>[2x]MTIYVVTPTYARLVQKAELVRLSQTLSLVPRLHWLLVEDAEGPTPLVSGLLAASGLLFTHLVVLTPKAQRLREGEPGWVHPRGVEQRNKALDWLRGRGGAVGGEKDPPPPGTQGVVYFADDDNTYSRELFEEMRWTRGVSVWPVGLVGGLRFEGPQVQDGRVVGFHTAWEPSRPFPVDMAGFAVALPLLLDKPNAQFDSTAPRGHLESSLLSHLVDPKDLEPRAANCTRVLVWHTRTE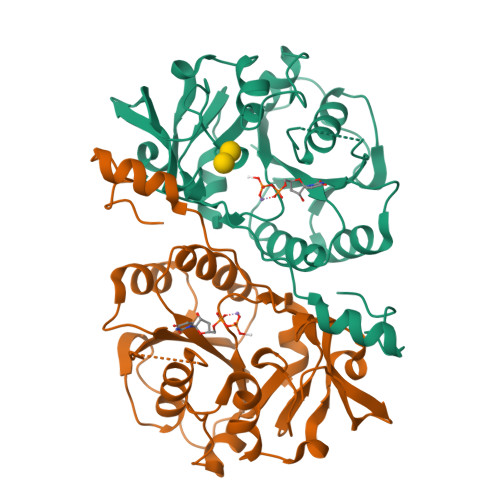KPKMKQEEQLQRQGRGSDPAIEV>[4x]GSHMSENFAVATPVRVGIVGTGYAAQRRAEVFRGDRRSQLVSFWGNSEANTAKFADTFGVRPQQSWQALINDPEIDLVLIATINQLHGAIAEAALQAGKHVVLEYPLALTYAMGKKLQQLAREKGKLLHVEHIE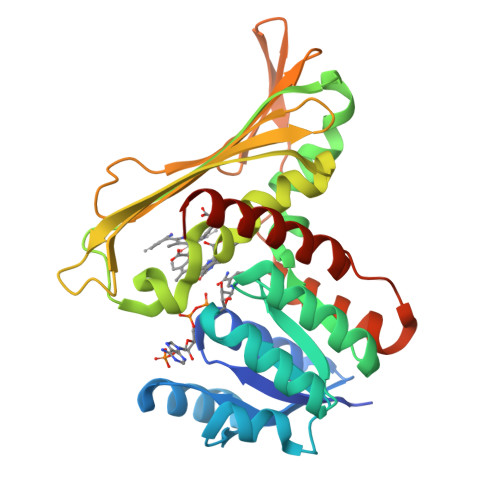LLGGVHQAIRQNLGKIGEVFYARYSTIMGQNPAPQRWTYHHQQFGFPLVAALSRISRFTDLFGTVQQVDAQCRFWDQPNPEYFRACLATAYLQFNNGLKAEVIYGKGEVFHQNERIFTLHGDRGTLIFVGETGRLIQGQTETEITVGSRRGLFRQDTEAVLDYLTTGKPLYVDLEASLYALEVADLCAQACGYKVEN>[4x]GPHMAAASPPLLRCLVLTGFGGYDKVKLQSRPAAPPAPGPGQLTLRLRACGLNFADLMARQGLYDRLPPLPVTPGMEGAGVVIAVGEGVSDRKAGDRVMVLNRSGMWQEEVTVPSVQTFLIPEAMTFEEAAALLVNYITAYMVLFDFGNLQPGHSVLVHMAAGGVGMAA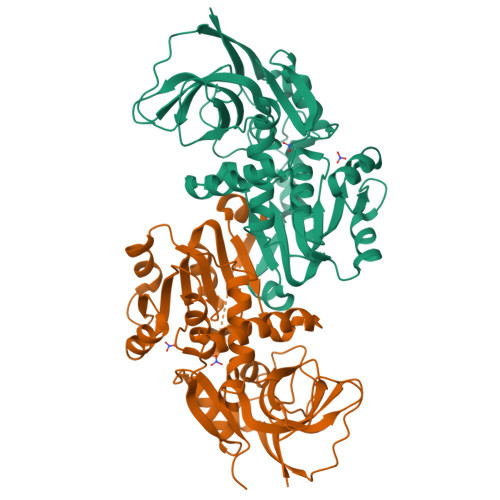VQLCRTVENVTVFGTASASKHEALKENGVTHPIDYHTTDYVDEIKKISPKGVDIVMDPLGGSDTAKGYNLLKPMGKVVTYGMANLLTGPKRNLMALARTWWNQFSVTALQLLQANRAVCGFHLGYLDGEVELVSGVVARLLALYNQGHIKPHIDSVWPFEKVADAMKQMQEKKNVGKVLLVPGPEKEN> VDCSEYPK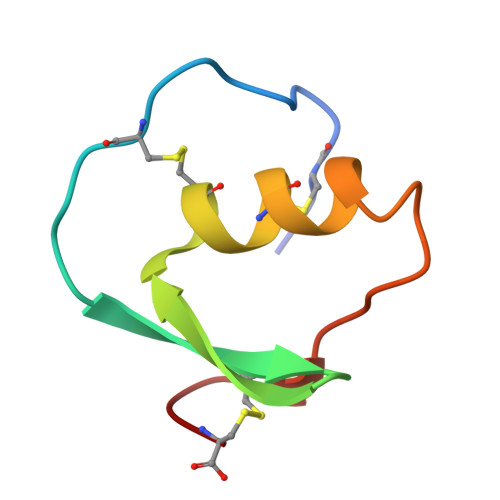PACTAEYRPLCGSDNKTYGNKCNFCNAVVESNGTLTLSHFGKC>QEGLDFPEYDGVDRVINVNAKNYKNVFKKYEVLALLYHEPPEDDKASQRQFEMEELILELAAQVLEDKGVGFGLVDSEKDAAVAKKLGLTEVDSMYVFKGDEVIEYDGEFSADTIVEFLLDVLEDPVELIEGERELQAFENIEDEIKLIGYFKSKDSEHYKAFEDAAEEFHPYIPFFATFDSKVAKKLTLKLNEIDFYEAFMEEPVTIPDKPNSEEEIVNFVEEHRRSTLRKLKPESMYETWEDDMDGIHIVAFAEEADPDGFEFLETLKAVAQDNTENPDLSIIWIDPDDFPL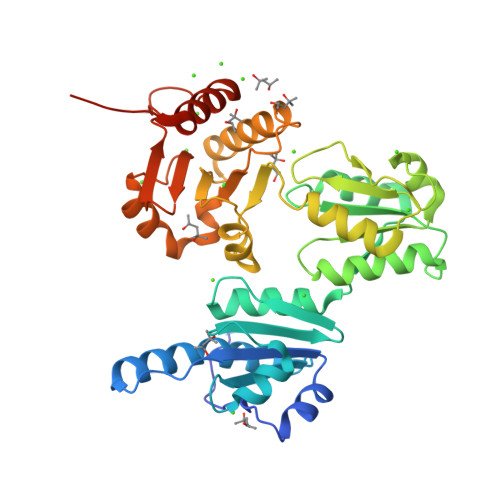LVPYWEKTFDIDLSAPQIGVVNVTDADSVWMEMDDEEDLPSAEELEDWLEDVLEGEINTEDDDDDDDD[6x]> MREMHHSRWSKIGTALAVSSALGLMSGMSVANDKLVELSKSNENWVMQGKDFSGTHYSTAKQINKDNVKKLRPSWSFSTGVLNGHEGAPLVVNGTMYIHTPFPNNTFAIDLDEPGVIKWEHKPKQDPAARAVACCDVVNRGLAYWPGDDKAPAMIVKSLLDGHVVALNAETGEEYWKVENGDISVGQTETAAPFVAKDLVIQGSSGAELGVRGYVTAYDIHTGEMVWRWYATGPDADVGLDKDFNKHNPHYGQKGLGTSTWEDNAWKIGGGTNWGWYAYDPQLDMFYYGSGNPAPWNETMRPGDNKWTMTIWGRDLETGLAKFGYQKTPHDEWDYAGVNVMMLSEQKDKNGKMRKLLTHPDRNGIIYTLDRETGDLVSANKMDDTANWVKKVDLETGLPIRDPEYG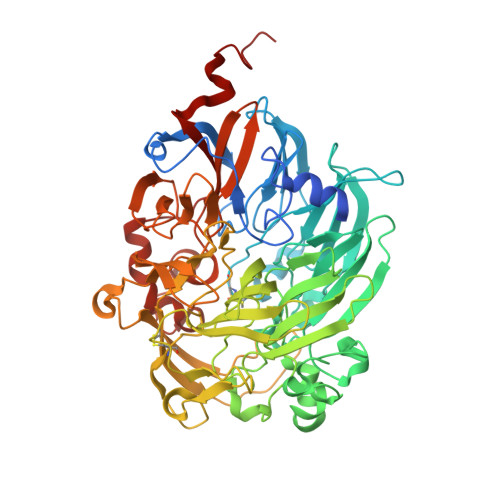TRMGHRSRDVCPSAMGFHNQGFDSYDPKRELFYLGINHLCMDWEPFMLPYRAGQFFVGANVWTYPGPKGDRQNGIGSGQVKAYNAITGEFAWEKMEKFSVWGGTTATEGGLVFYGTLDGFIKARDADTGKLLWKFKLPSGVIGHPMTYTHKGTQYVAINYGVGGWPAVGLVFDLNDPSAGLGAVGAFKELAKNTQMGGGVMVFSLDGKSPYDDVSLGEYGM> QQYECVAEIGEGAYGKVFKARDLKNGGRFVALKRVRVQTGEEGMPLSTIREVAVLRHLETFEHPNVVRLFDVCTVSRTDRETKLTLVFEHVDQDLTTYLDKVPEPGVPTETIKDMMFQLLRGLDFLHSHRVVHRDLKPQNILVTSSGQIKLADF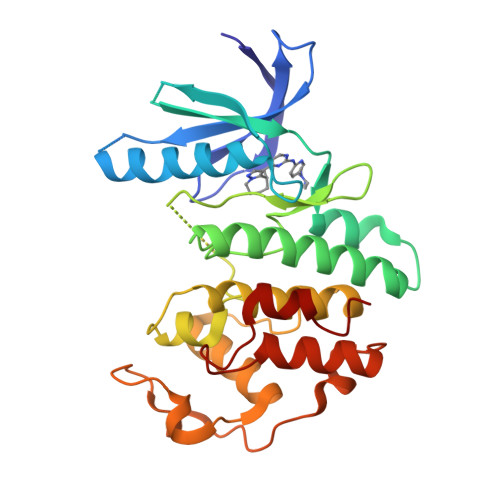GLARIYSFQMALTSVVVTLWYRAPEVLLQSSYATPVDLWSVGCIFAEMFRRKPLFRGSSDVDQLGKILDVIGLPGEEDWPRDVALPRQAFHSKSAQPIEKFVTDIDELGKDLLLKCLTFNPAKRISAYSALSHPYFQ>[2x]MDHLPIFCQLRDRDCLIVGGGDVAERKARLLLEAGARLTVNALTFIPQFTVWANEGMLTLVEGPFDETLLDSCWLAIAATDDDTVNQRVSDAAESRRIFCNVVDAPKAASFIMPSIIDRSPLMVAVSAGGTSPVLARLLREKLESLLPQHLGQVARYAGQLRARVKKQFATMGERRRFWEKFFVNDRLAQSLANADEKAVNATTERLFSEPLDHR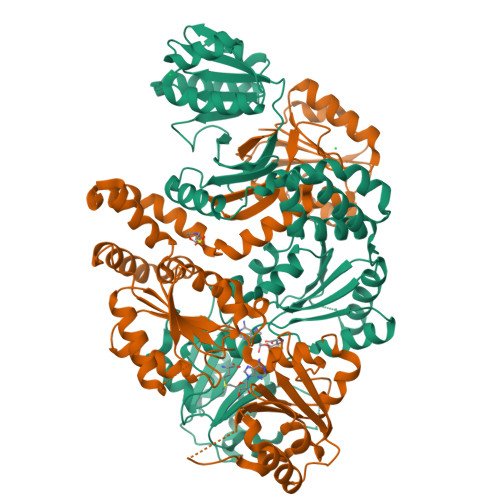GEVVLVGAGPGDAGLLTLKGLQQIQQADIVVYDRLVSDDIMNLVRADADRVFVGKRAGYHCVPQEEINQILLREAQKGKRVVRLKGGDPFIFGRGGEELETLCHAGIPFSVVPGITAASGCSAYSGIPLTHRDYAQSVRLVTGHLKTGGELDWENLAAEKQTLVFYMGLNQAATIQEKLIAFGMQADMPVALVENGTSVKQRVVHGVLTQLGELAQQVESPALIIVGRVVALRDKLNWFSNH> GPGSTSAVLLDHCHFSQVIFNSVEKFYIPGGDVTCHYTFTQHFIPRRKDWIGIFRVGWKTTREYYTFMWVTLPIDLNNKSAKQQEVQFKAYYLPKDDEYYQFCYVDEDGV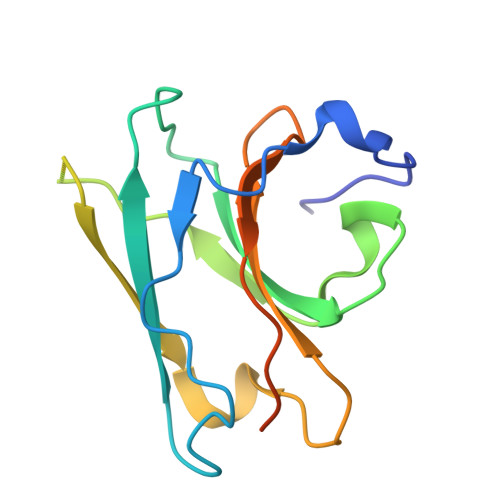VRGASIPFQFRPENEEDILVVTTQGE>[2x]MGSHHHHHHSQDSVTIFILSVIHVKPPFKLKRKFQNNPHYEKEMRRQLKMQEDGINKLTVFEWLTNRKTFREKGRLSSQTAQNDARDAYKRRKMFDYMLLSAENFKYDEITKKVEDELSSLAALHNPDQIAGGNFDDVTAMGDKRINSSIGSQWGTKDKGRAQNLED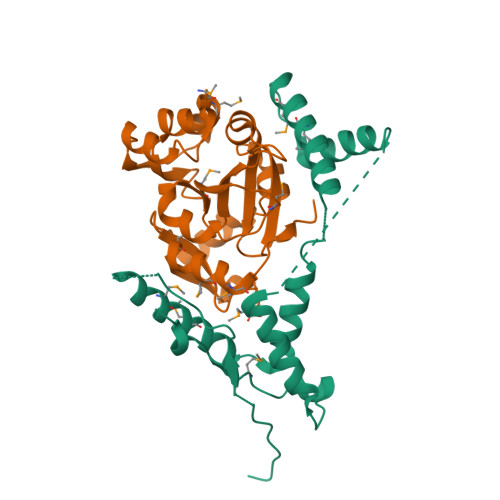ELLKVLEGPPKIDEEQQKYIKMNVIFAEDLEIIK;>[2x]MYEMFLFNSVNSKITQNVNEEFILKYSDYSCEQLNSLWKEVGLGSYYNGLFKIIEPNDLKDIINQCYIMDDDESLLPFMCTAFGDVFAYVKNKRFGNYVVFLNIRYGTSLIIPDNFVAIFNKVIPNQSFLKGWFDLENYAFVKEKIGEIDFDECYGYFPTLSMGGNESIDNISIVKMIPYIDMNVQMIDVFERADKHHHHHH>[2x]DDKAACADGIAAVKARVEKLAPEAVPQKLKRALKIAEREQ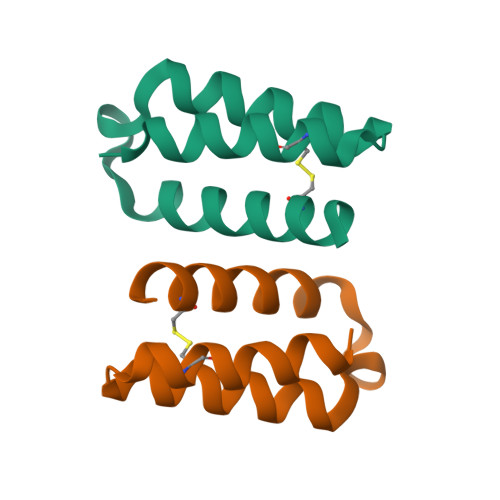GEGEFDECLEALDDAKRALPK> MAGTALKRLMAEYKQLTLNPPEGIVAGPMNEENFFEWEALIMGPEDTCFEFGVFPAILSFPLDYPLSPPKMRFTCEMFHPNIYPDGRVCISILHAPGDDPMGYESSAERWSPVQSVEKILLSVVSMLAEPNDESGANVDASKMWRDDREQFYKIAKQIVQKSLGL;> HMKNYLRVVGNMEARFAVATPEE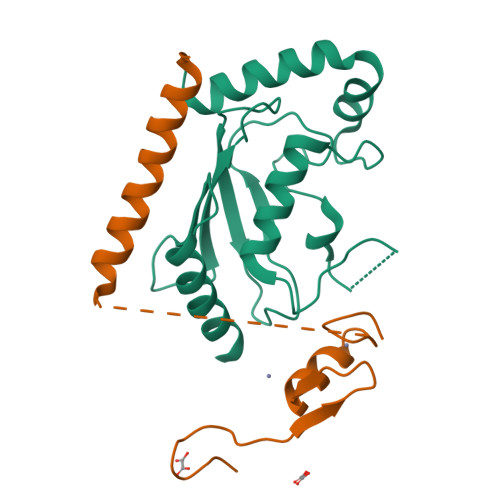LAVNNDDCAICWDSMQAARKLPCGHLFHNSCLRSWLEQDTSCPTCRMSLNIADNNRVREEGGGGGGGSSGSSGGSGGGSGSSSGGGGGSGGGSGGGGGGGSADERQRMLVQRKDELLQQARKRFLNK In the T4SS from the enterococcal conjugative plasmid pCF10, PrgK is known to be the active cell wall degrading enzyme. It has three predicted extracellular hydrolase domains: metallo-peptidase (LytM), soluble lytic transglycosylase (SLT), and cysteine, histidine-dependent amidohydrolases/peptidases (CHAP). The pCF10-encoded PrgK is essential for conjugation and belongs to the DELTA family of larger PG-degrading enzymes. To conclude, we here show that PrgK, an essential cell wall degrading enzyme of the pCF10 T4SS, has muramidase activity instead of the lytic transglycosylase activity that has been shown for other T4SS cell wall degrading enzymes.

Therefore, we directed our efforts toward the extracytoplasmic region (PrgKEC), as well as its individual LytM, SLT, and CHAP domains. Crystallization trials yielded crystals of the PrgKLytM domain, which were used to solve the LytM structure to 1.5 Å. In agreement with bioinformatic predictions, our crystal structure confirms that the active site of LytM is degenerate as it lacks the conserved HXXXD and HXH motifs required for zinc ion coordination at the catalytic site. This is not the only characterized LytM domain with a degenerate active site. Sequence alignment of PrgKLytM homologs shows very low sequence identity, with only the region encompassing the HXXXD and HXH motifs being conserved. The His and Asp residues that are important for catalysis are only conserved in active homologs, but not in PrgKLytM and other degenerate homologs. The crystal structure of LytM superimposes well onto the AF model with an r.m.s.d. of 0.43 Å. Only one structural homolog was found in the PDB by using Foldseek, which is the geneproduct 13 (gp13) cell-wall degrading enzyme of bacteriophage Φ29 (54). gp13 consists of two domains, one N-terminal lysozyme-like domain that is homologous to the MUR domain (RMSD of 1.5 Å), and a C-terminal LytM domain (RMSD to PrgKLytM of 2.4 Å). However, the muropeptide profiles of the PrgKSLT-CHAP:C766A, H828A and PrgKEC:C766A, H828A fractions after incubation with cell-wall extract are similar to their wild-type counterparts. In line with this result, the LytM and CHAP domains showed no activity against the sacculi. In conclusion, the LytM domain of PrgK has a degenerate active site and might play a regulatory role.

>[2x]GPSASSTQKPAIVQEEEDLTASWTYFTKLDAQHTDDNNLFYSNIDEVLFYMNYRYDDFKLLDMDSTGTKNFETILSELWTALNGKKPDYQLKTMQSLETDKKSSYFIEEEQAKHYQEIKKELGYQTLDDLLSFPVKTDALIVNKRYGYDKSKEKLTLYQGIDVLIEDNQPFHSPMNGQIVSVPDTETLVIEKEKVARLTIRGVNTLRLTKGMDVEEGTFLGNTKNSTVTFQYEKYKKETKDWFFVNPAFYFPRVTYTQTTA{2-[(3S)-3-(2-amino-6-oxo-1,6-dihydro-9H-purin-9-yl)pyrrolidin-1-yl]-2-oxoethyl}phosphonic acid | C11 H15 N6 O5 P | 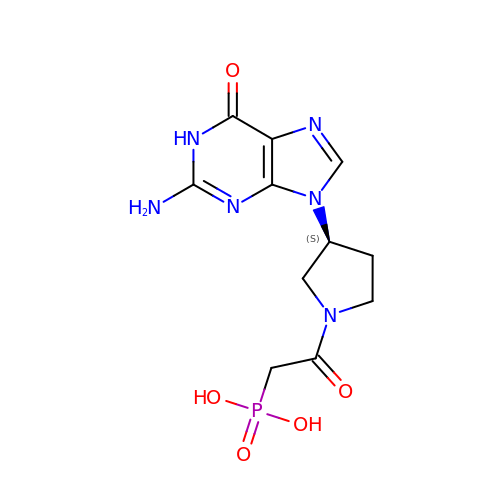DPSMTUGMQGDYNX-LURJTMIESA-N> QFAKPEDAVKYRQS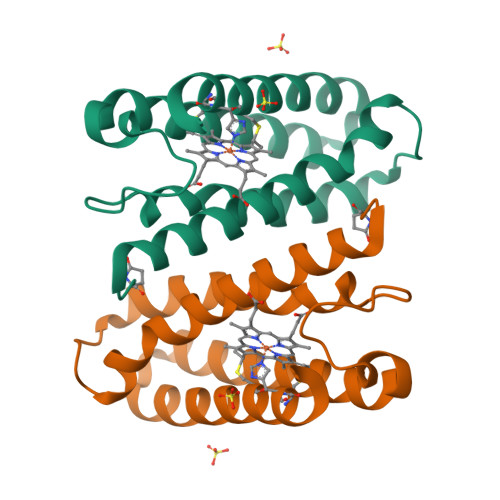ALTLMASHFGRMTPVVKGQAPYDAAQIKANVEVLKTLSALPWAAFGPGTEGGDARPEIWSDAASFKQKQQAFQDNIVKLSAAADAGDLDKLRAAFGDVGASCKACHDAYQKKK> AALRERAGPVTWVMMIACVVVFIAMQILGDQEVMLWLAWPFDPTLKFEFWRYFTHALMHFSLMHILFNLLWWWYLGGAVEKRLGSGKLIVITLISALLSGYVQQKFSGPWFGGLSGVVYALMGYVWLRGERDPQSGIYLQR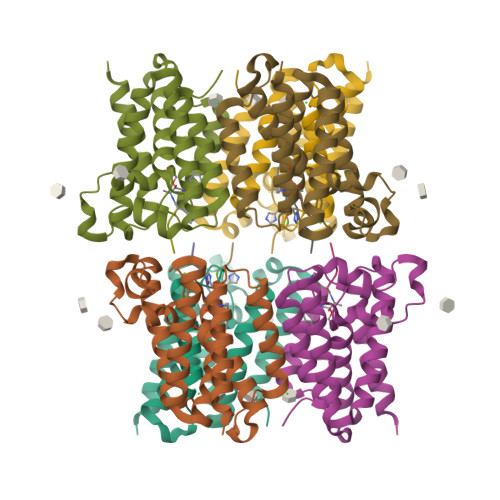GLIIFALIWIVAGWFDLFGMSMANGAHIAGLAVGLAMAFVDSLNARKRK>MPLGLLWLGLALLGALHAQAQDSTSDLIPAPPLSKVPLQQNFQDNQFQGKWYVVGLAGNAILREDKDPQKMYATIYELKEDKSYNVTSVLFRKKKCDYWIRTFVPGSQPGEFTLGNIKSYPGLTSYLVRVVSTNYNQHAMVFFKKVSQNREYFKITLYGRTKELTSELKENFIRFSKSLGLPE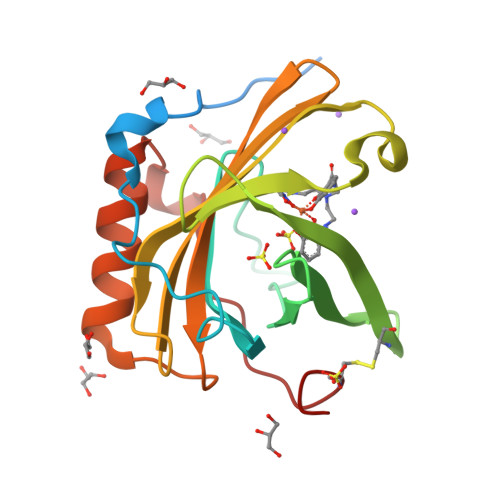NHIVFPVPIDQCIDG[3x]> FHV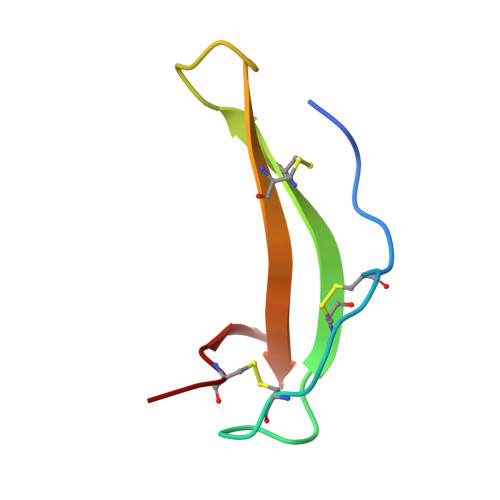PDDRPCINPGRCPLVPDATCTFVCKAADNDFGYECQHVWTFEGQRVGCYA N-(phenylmethyl)pyridin-2-amine | C12 H12 N2 | 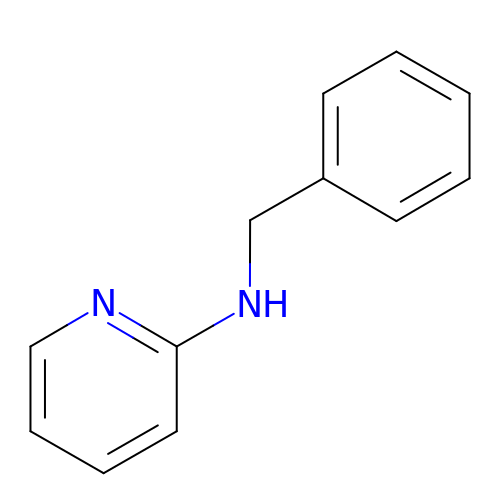WYHXNQXDQQMTQI-UHFFFAOYSA-N>[2x]MGIRITGTGLFHPTEIISNEELADSLNAYVEQYNQENAEKIAAGELEELRGSSAEFIEKASGIKRRYVIEKSGILDPTRLRPRLSERSNDELSIQAEWGVIAAKQAMENAGVTAEDIDVVILACSNM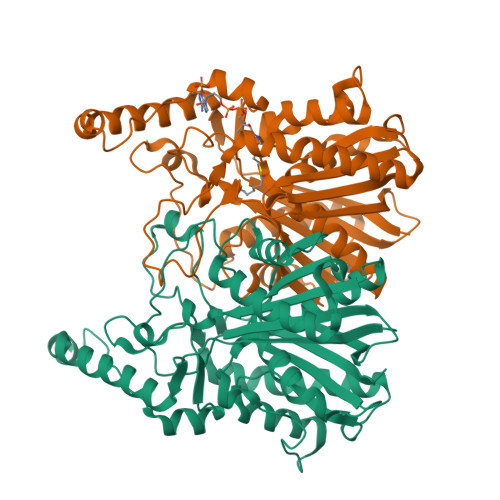QRAYPAVAIEIQSALGIQGYAYDMNVAASAATFGLKQAADAIRSGARRVLLVNVEITSGHLDYRNRDCHFIFGDVATASIIEETTTKTGFEILDIHLFTQFSNNIRNNFGFLNRSEDAVVDDKLFRQDGRKVFKDVAPLVAKIINAQLEKMQLTANDIKRFWLHQANANMNELILKYVAGKDADLSRAPIILDEFANTSSAGVIIALHRTGHEVDDGEYGVISSFGAGYSVGSIVVQKHVA> GHMKQEELKRLYKAQAIQRQLEEVEERQRASEIQGVRLEKALRGEADSGTQDEAQLLQEWFKLVLEKNKLMRYESELLIMAQELELEDHQSRLEQKLREKMLKEESQKDEKDLNEEQEVFTELMQVIEQRDKLVDSLEEQRIREKAEDQHFES;> GHMNPEYDYLFKLLLIGDSGVGKSCLLLRFADDTYTESYISTIGVDFKIRTIELDGKTIKLQIWDTAGQERFRTITSSYYRGAHGIIVVYDVTDQESYANVKQWLQEIDRYASENVNKLLVGNKSDLTTKKVVDNTTAKEFADSLGIPFLETSAKNATNVEQAFMTMAAEIKKRMGPGAASGGERPNLKIDSTPVKPAGGGCC

Rab proteins, the biggest subfamily within the superfamily of small GTPases, are major regulators of vesicular trafficking in eukaryotic cells. One such family of effector proteins that was reported to link Rab proteins and the cytoskeleton is the Mical (molecules interacting with CasL) family. In this publication, we present a thorough biochemical and structural analysis of a Rab effector domain termed bivalent Mical/EHBP Rab binding (bMERB) domain. The results show that the domains probably constitute a Rab8-effector family involved in endosomal trafficking, and the Rab-binding specificity can be well explained from the 3-dimensional structures of complexes determined in this work.

Well diffracting crystals were found using the RBD of Mical-cL (residues 534–683) in complex with different Rab proteins (Rab1, Rab8 and Rab10). In all structures (Rab1:Mical-cL, Rab8:Mical-cL and Rab10:Mical-cL) we found one Rab protein bound to one molecule of Mical-cL, in agreement with the previous observations that all Rab proteins tested bind only one site in Mical-cL. Most interactions were visible between the Rab proteins and α-helix 3 of Mical-cL with some additional contributing residues from α-helix 2, forming extensive contacts involving residues within switch I and II of the Rab proteins. Since the interacting residues in the RabSF1 and RabSF2 regions are strongly conserved between both Rab1 and Rab8 families, this did not explain the observed preference of the RBD towards the Rab8 family. However, we observed that the main chain atoms of the N-terminal residues preceding the RabSF1 motif can be traced in the electron density and seem to interact with amino acids within α-helix 1 and 2 of Mical-cL, even though the electron density in this region did not allow a precise localization of the side chains. In contrast to the main interacting helix α3, which adopts a similar position in all three structures, we observed slightly different orientations of the α-helices 1 and 2, adopting a position slightly further away from Rab1 compared to Rab8 and Rab10. Interestingly, whereas Rab1 contains a glutamate near the N-terminus (Glu4), all Rab8 family members contain one or (in the case of Rab10) two lysine residues in this region that point towards a negatively charged patch in Mical-cL. Consistently, the negatively charged N-terminus of Rab1 seems to repel α-helices 1 and 2 of Mical-cL and they adopt a conformation slightly further away from Rab1 compared to Rab8 and Rab10 (also see (a)). Using Mical-cL as one representative of the bMERB family, we saw that all members of the Rab8 family bound Mical-cL with high nanomolar affinities, compared to Rab1 (KD = 5.2 µM) and Rab35 (KD = 1.8 µM).> GMSSKRLVIVGGGITGLAAAYYAERAFPDLNITLLEAGERLGGKVATYREDGFTIERGPDSYVARKHILTDLIEAIGLGEKLVRNNTSQAFILDTGGLHPIPKGAVMGIPTDLDLFRQTTLLTEEEKQEVADLLLHPSDSLRIPEQDIPLGEYLRPRLGDALVEKLIEPLLSGIYAGNIDQMSTFATYPQFVANEQKAGSLFEGMRLMRPLDQLPQTPQTTIKATGQFLSLETGLESLIERLEEVLERSEIRLETPLLAISREDGRYRLKTDHGPEYADYVLLTIPHPQVVQLLPDAHLPELEQL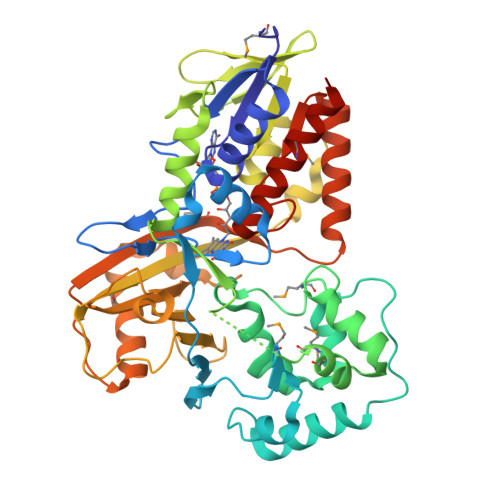TTHSTATVTMIFDQQQSLPIEGTGFVVNRRAPYSITACTAIDQKWNHSAPDHTVLRAFVGRPGNDHLVHESDEVLQQAVLQDLEKICGRTLEPKQVIISRLMDGLPAYTVGHADRIQRVREEVLAQYPGIYLAGLAYDGVGLPDCVASAKTMIESIELEQSHTDESVNET N-propargylglycine-modified flavin adenine dinucleotide | C32 H40 N10 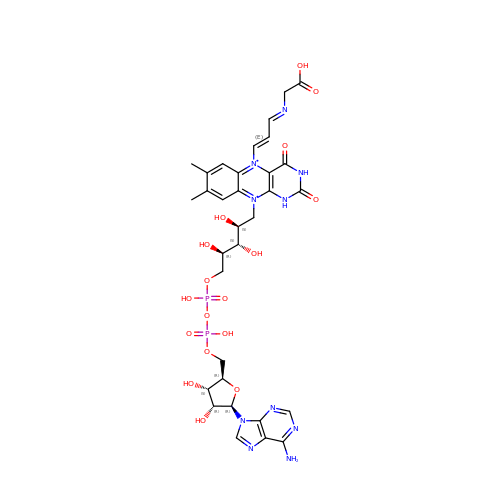O17 P2 | IRSTVKNHNHEQIM-RDJFLKOLSA-N O-phosphono-N-(5-sulfanylpentanoyl)-L-threonine | C9 H18 N O7 P S 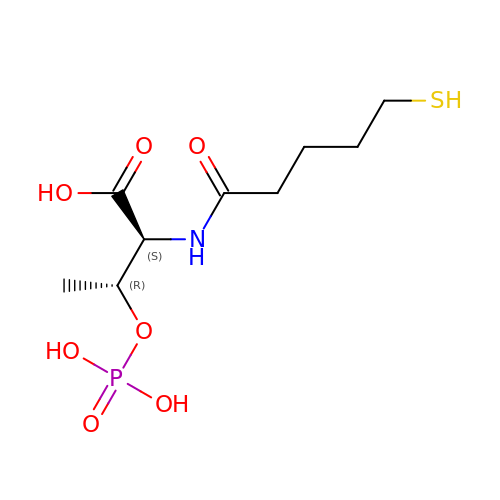| PXLGZPNRHROFQI-SVRRBLITSA-N> XAD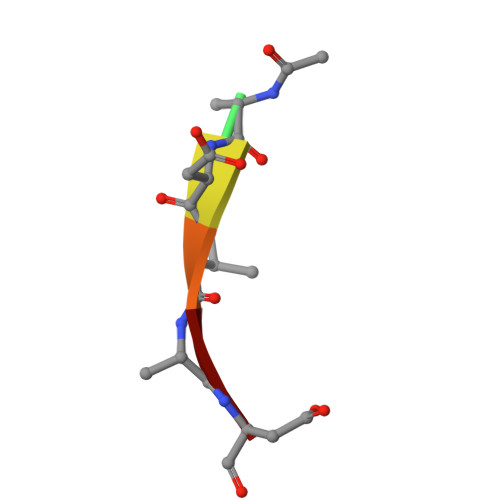VAD>[2x]TDLPRPSISAEPGTVI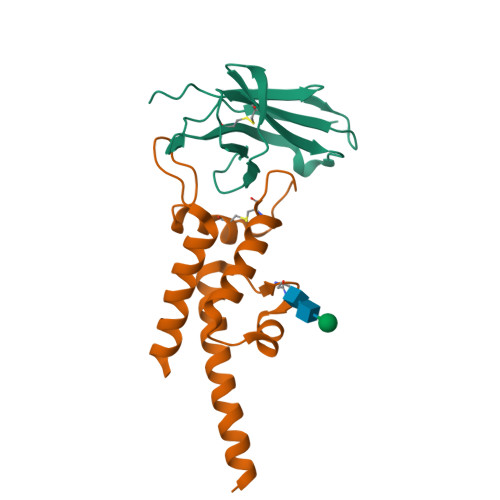PLGSHVTFVCRGPVGVQTFRLERERNYLYSDTEDVSQTSPSESEARFRIDSVNAGNAGLFRCIYYKSRKWSEQSDYLELVVKGEDVTWA;>TDAIAAATKAAMIEGAAQGAVAGEAAGRNAIIGALKRYFHIDNLNGTSLKSFFNSTSYSDVTTIASAIDTQMTASCDAFSGKIVNQAFCDVRKTLRIVADPGKSFVKQKDAITGAVTQLVEKAKDTASFKATEVSSATSSKIITKQNALIE[2x]>MDHRTSIAQAMVDRISKQMDGSQPDEYFNNLYGNVSRQTYKFEEIREFPYVAVHIGTETGQYLPSGQQWMFLELPILVYDKEKTDIQEQLEKLVADIKTVIDTGGNLEYTVSKPNGSTFPCEATDMIITSVSTDEGLLAPYGLAEINVTVRYQPPRRSLRR[6x];>[3x]MSLQLLRNTRIFVSTVKTGHNKTNTQEILVQDDISWGQDSNSTDITVNEAGPRPTRGSKRFNDSLNAAEWSFSTYILPYKDKNTSK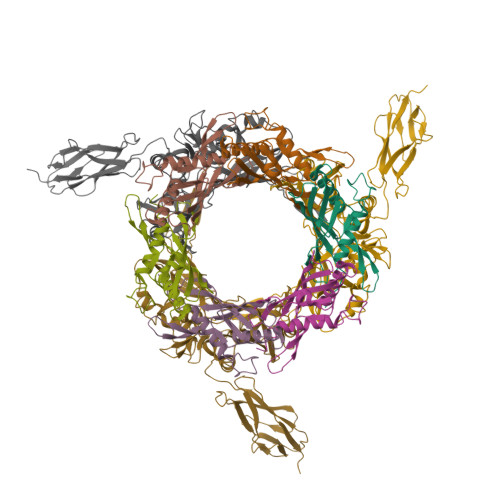QIVPDYMLWHALSSGRAINLEGTTGAHNNATNFMVNFKDNSYHELAMLHIYILTDKTWSYIDSCQINQAEVNVDIEDIGRVTWSGNGNQLIPLDEQPFDPDQIGIDDETYMTIQGSYIKNKLTILKIKDMDTNKSYDIPITGGTFTINNNITYLTPNVMSRVTIPIGSFTGAFELTGSLTAYLNDKSLGSMELYKDLIKTLKVVNRFEIALVLGGEYDDERPAAILVAKQAHVNIPTIETDDVLGTSVEFKAIPSDLDAGDEGYLGFSSKYTRTTINNLIVNGDGATDAVTAITVKSAGNVTTLNRSATLQMSVEVTPSSARNKEVTWAITAGDAATINATGLLRADASKTGAVTVEATAKDGSGVKGTKVITVTAGG>MGEYEGGSNDFVYSIWKGPVIRAGNFALHPEVVREEVKDKRTLIGYGRFFISNPDLVDRLEKGLPLNKYDRDTFYQMSAHGYIDYPTYEEALKLGWGTSSFVKDFKPQALGDTNLFKPIKIGNNELLH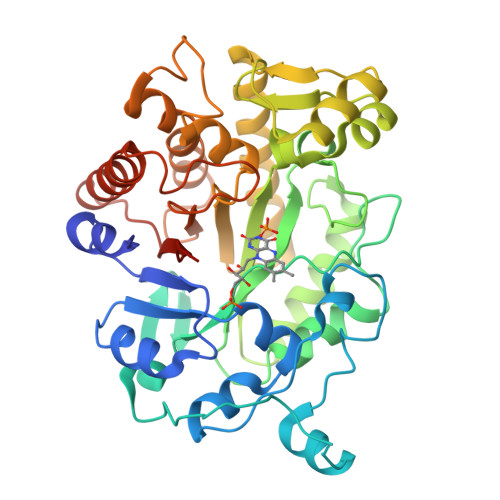RAVIPPLTRMRALHPGNIPNRDWAVEYYTQRAQRPGTMIITEGAFISPQAGGYDNAPGVWSEEQMVEWTKIFNAIHEKKSFVWVQLWVLGWAAFPDNLARDGLRYDSASDNVFMDAEQEAKAKKANNPQHSLTKDEIKQYIKEYVQAAKNSIAAGADGVEIHSANGYLLNQFLDPHSNTRTDEYGGSIENRARFTLEVVDALVEAIGHEKVGLRLSPYGVFNSMSGGAETGIVAQYAYVAGELEKRAKAGKRLAFVHLVEPRVTNPFLTEGE[4x]> SNAMNLFTRHRNNIRLTTAGEKLLPYAETLMNTWQAARKEVAHSSRHNEFSIGASASLWECMLNGWLGTLYSAPYNLQFEARIAQRQSLVKQLHERQLDLLITTESPKMDELSSQLLGNFTLALYCASPAKNRNELNYLRLEWGPDFQQNEVGLIGSDDVPLLTTSSAELIYQQLSRLNGCCWLPARWAKEKHGLHTVMDSATLSRPLYAIWLQNSDKQAQIHEILKNPILE

Here, we report the deposition of 14 structures of enzymes from both the core and accessory genomes of sequence type 23 (ST23) K1 hypervirulent K. pneumoniae. Targets were selected using a shotgun approach aimed at uncharacterized metabolic proteins from ST23 K1 hypervirulent K. pneumoniae. In silico multilocus sequence typing of all K. pneumoniae isolates was completed using Kleborate. This analysis showed that 64 of the selected proteins are part of the K. pneumoniae core genome, defined as genes present in at least 95% of all strains; the other 132 proteins are part of the K. pneumoniae accessory genome and are overrepresented in the highly virulent hvKp clonal group CG23, which contains ST23 (7). Thus, the x-ray crystal structures presented here provide the basis for functional analysis of 12 uncharacterized proteins associated with high-risk K. pneumoniae infection.

In all, structures represent both metabolic proteins and possible transcriptional regulators.> MASMTGGQQMGRDEAGITGTWYNQLGSTFIVTAGADGALTGTYESAVGNAESRYVLTGR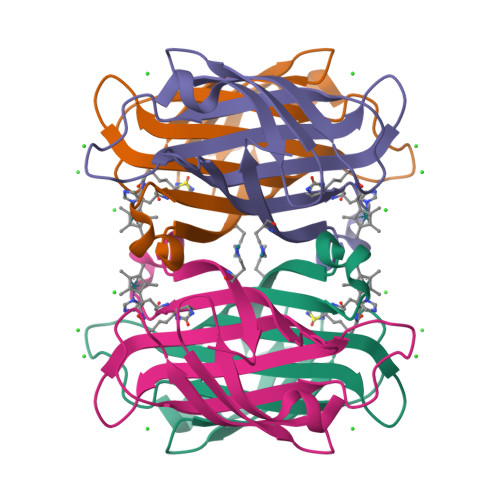YDSAPATDGSGTALGWTVAWKNNYRNAHSATTWSGQYVGGAEARINTQWLLTHGTTEANAWKSTLVGHDTFTKVKPSAASIDAAKKAGVNNGNPLDAVQQ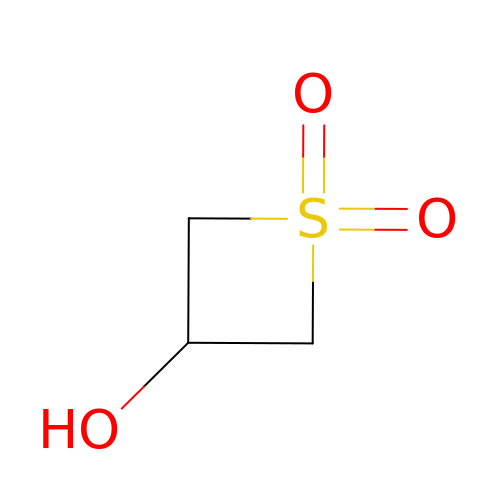1,1-bis(oxidanylidene)thietan-3-ol | C3 H6 O3 S | CIUZABLJPXPIFC-UHFFFAOYSA-N>[2x]CG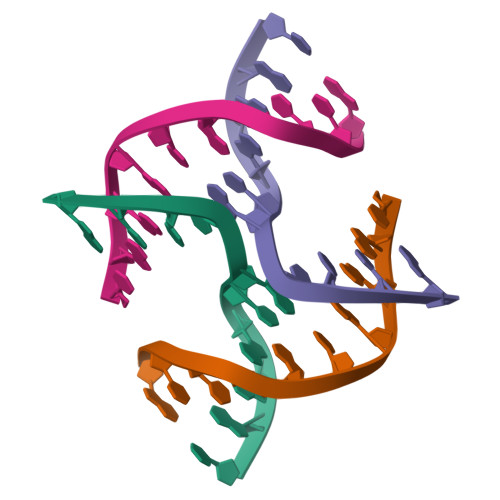GGCGCCCG>DRLFNVVARGNPEDLAGLLEYLRRTSKYLTDSEYTEGSTGKTCLMKAVLNLQDGVNACIQPLLEIDRDSGNPQPLVNAQCTDEYYRGHSALHIAIEKRSLQCVKLLVENGANVHAKACGHFFQKNQDTCFYFGELPLSLAACTKQWDVVNYLLENPHPAASLQAQDSLGNTVLHALVMIADNSPENSALVVRMYDGLLQAGARLCPNVQLEGIPNLEGLTPLKLAAKEGKIEIFKHILQREFSAPCQSLSRKFTEWCYGPVRVSLYDLASVDSWEENSVLEIIAFHSRSPHRHRMVVLEPLNKLLQAKWDRLIPRFCFNFLCYLVYMLIFTAVAYHQPALEKQGFPPLKATAGNSMLLLGHILILLGGVYLLLGQLWYFWRRRLFIWISFMDSYFEILFLLQALLTVLSQVLCFLAIEWYLPLLVSSLVLGWLNL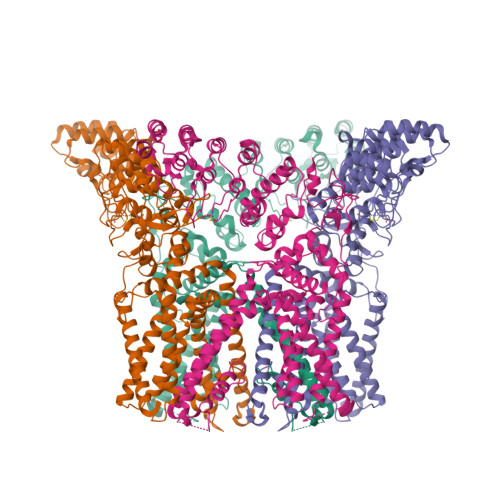LYYTRGFQHTGIYSVMIQKVILRDLLRFLLVYLVFLFGFAVALVSLSREAQEDEAPPYRSILDASLELFKFTIGMGELAFQEQLRFRGVVLLLLLAYVLLTYVLLLNMLIALMSETVNSVATDSWSIWKLQKAISVLEMENGYWWCRRKKQRAGVMLTVGTRPDGSPDERWCFRVGEM[4x]>MSQHNEKNPHQHQSPLHDSSEAKPGMDSLAPEDGSHRPAAEPTPPGAQPTAPGSLKAPDTRNEKLNSLEDVRKGSENYALTTNQGVRIADDQNSLRAGSRGPTLLEDFILREKITHFDHERIPERIVHARGSAAHGYFQPYKSLSDITKADFLSDPNKITPVFVRFSTVQGGAGSADTVRDIR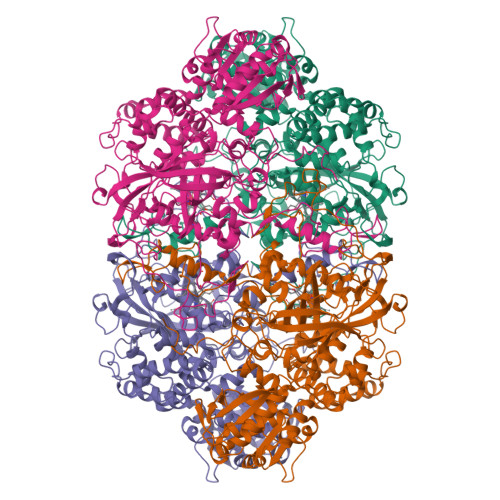GFATKFYTEEGIFDLVGNNTPIFFIQDAHKFPDFVHAVKPEPHWAIPQGQNAHDTFWDYVSLQPETLHNVMWAMSDRGIPRSYRTMEGFGIHTFRLINAEGKATFVRFHWKPLAGKASLVWDEAQKLTGRDPDFHRRELWEAIEAGDFPEYELGFQLIPEEDEFKFDFDLLDPTKLIPEELVPVQRVGKMVLNRNPDNFFAENEQAAFHPGHIVPGLDFTNDPLLQGRLFSYTDTQISRLGGPNFHEIPINRPTCPYHNFQRDGMHRMGIDTNPANYEPNSINDNWPRETPPGPKRGGFESYQERVEGNKVRERSPSFGEYYSHPRLFWLSQTPFEQRHIVDGFSFELSKVVRPYIRERVVDQLAHIDLTLAQAVAKNLGIELTDDQLNITPPPDVNGLKKDPSLSLYAIPDGDVKGRVVAILLNDEVRSADLLAILKALKAKGVHAKLLYSRMGEVTADDGTVLPIAATFAGAPSLTVDAVIVPCGNIADIADNGDANYYLMEAYKHLKPIALAGDARKFKATIKIADQGEEGIVEADSADGSFMDELLTLMAAHRVWSRIPKIDKIPA[4x]>[6x]LSNEVSTDEALLKRYRKEIMDLKKQLEEVSLETRAQAMEKDQLEKER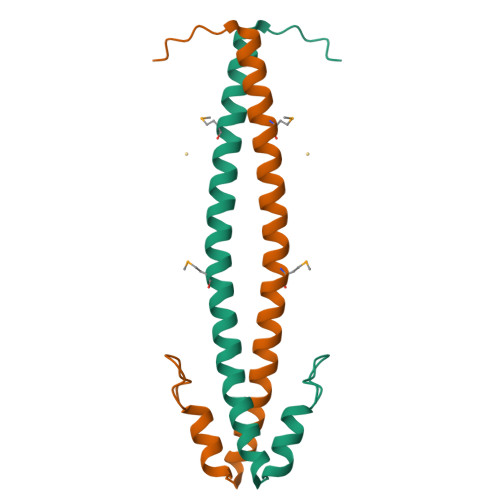DFYFGKLRNIELICQENEGENDPVLQRIVDILYATDEGFVIPD(3E)-3-{(1S,4S,4aS,5R,8aS)-1-[(2E,4R,7S,8E,10S)-1,7-dihydroxy-10-{(2R,3S,5R)-5-[(1S)-1-methoxyethyl]-3-methyloxolan-2-yl}-4-methylundeca-2,8-dien-2-yl]-4,5-dimethyloctahydro-3H-2-benzopyran-3-ylidene}oxolane-2,4-dione 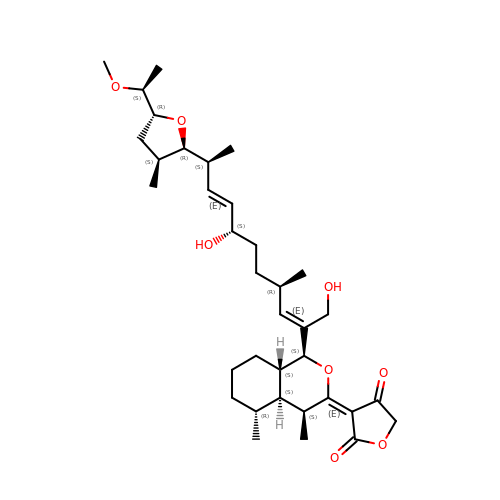| C35 H54 O8 | RLWRBBXSBCBSGG-HASGRZBRSA-N>[6x]MH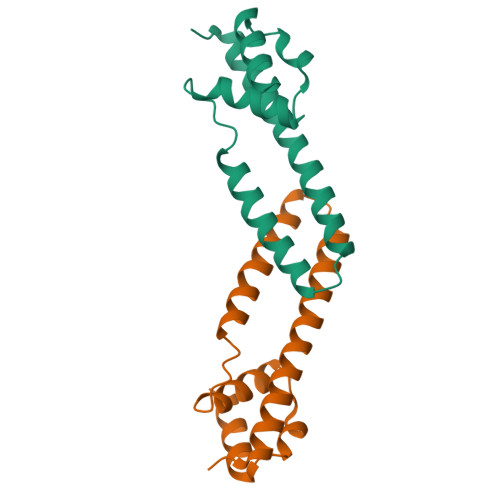HHHHHLQTAEAPWSQAETQSAHALFRKAYQRELDGLLATVQAQASQITQIDDLWKLHDFLSAKRHEIDGKYDDRQSVIIFVFAQLLKEGLVQAEELTFLAADKQSKIKALARL> HHHHHHSSVVVDTNGQPVSNGADAYYLVPVSHGHAGLALAKIGNEAEPRAVVLDPHHRPGRPVRFESPLRINIIKESYFLNIKFGPSSSDS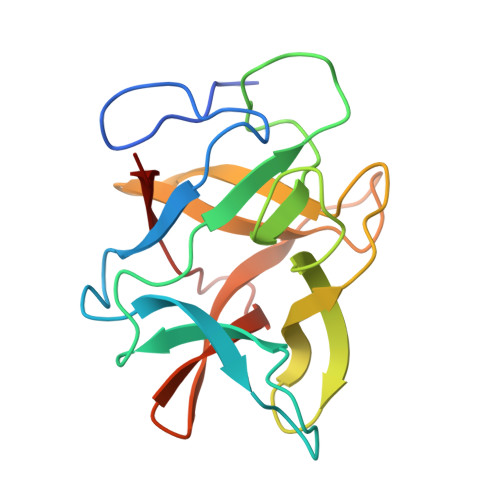GVWDVIQQDPIGLAVKVTDTKSLLGPFKVEKEGEGYKIVYYPERGQTGLDIGLVHRNDKYYLAVKDGEPCVFKIRKAT> GHMRERYELSEKMLSACNLLKNTINDPKALTSKDMRFCLNTLQHEWFRVSSQKSAIPAMVGDYIAAFEAISPDVLRYVINLAD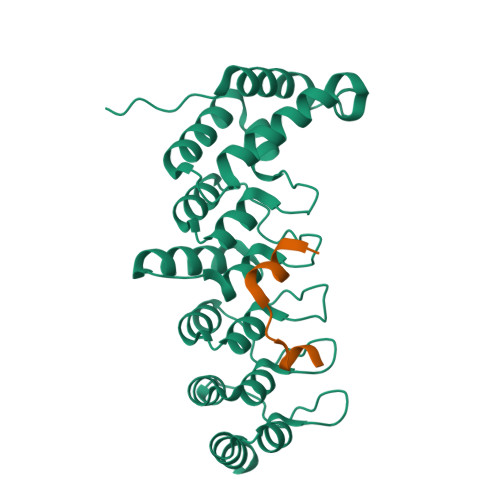GNGNTALHYSVSHSNFEIVKLLLDADVCNVDHQNKAGYTPIMLAALAAVEAEKDMRIVEELFGCGDVNAKASQAGQTALMLAVSHGRIDMVKGLLACGADVNIQDDEGSTALMCASEHGHVEIVKLLLAQPGCNGHLEDNDGSTALSIALEAGHKDIAVLLYAHVNFAKA;> EVKPKNKARRRTTTQMELLYAD4-[(2-fluorophenyl)methyl]-4,5-dihydropyrazin-2(3H)-one 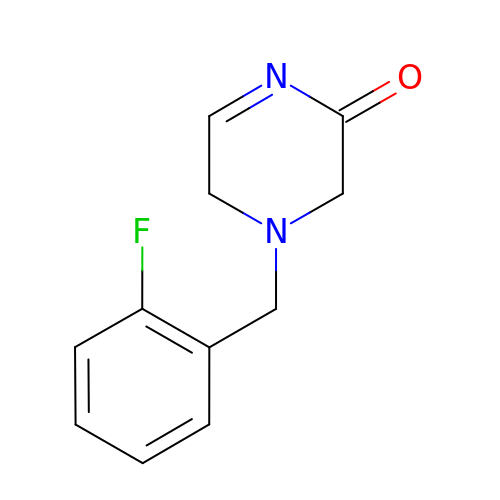| C11 H11 F N2 O | CFVZNWNMKVRFMY-UHFFFAOYSA-N> MAHHHHHHMAKTRVETDSMGEIEVPSDKYWGAQTERSLHHFNIGKDIMPREVTHAFGILKKAAALTNLELGKLPKDKADLIVQAAEEVSKGLLDEHFPLHVWQTGSGTQSNMNANEVISNRAIELAGGTLGSKSPIHPNDHVNMSQSSNDTFPTAMHIAAAIAFNEKLLPAVR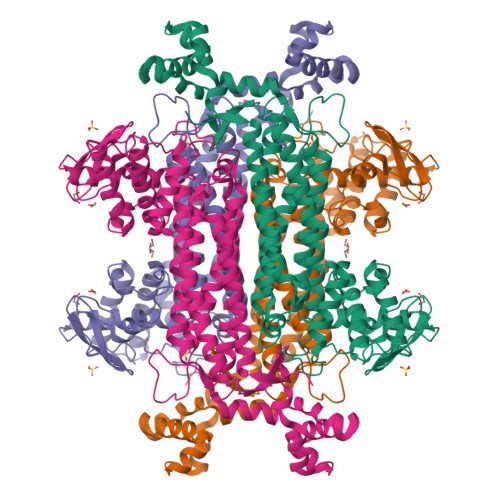NLRHVFAAKMDAFKNIIKIGRTHLQDAVPLTLGQEFSGYVAQLDACVHRLEEVLPELYELAAGGTAVGTGLNTHPQFAVKVAEHIAKITKLPFVTAPNKFAALASHEPLVHAHGAMKTLACALMKIANDIRWLASGPRCGIGELIIPENEPGSSIMPGKVNPTQCEAMTMVCAQVLGNDTAVGIADSQGNFELNVFKPVIIFNVLHSLNLLADSCHSFQEFCAEGIEPNQPVIDYYLHHSLMLVTALNQHIGYDKAAKIAKTAHHDNISLQEAAVKLGILTAEQFAEFVKPEKMISPEQ> MLVSCIRRQADRRTRHHMMLDGQINPREWMNWHPKEYQPWYFDRHKFLYERQQYAHFHHLLCHQVFLKDMLHLVQHPEPYTHIVDCRTSPLKMHRWVPHSWWLPRDEVEYALQLTPDEFADMYGFHK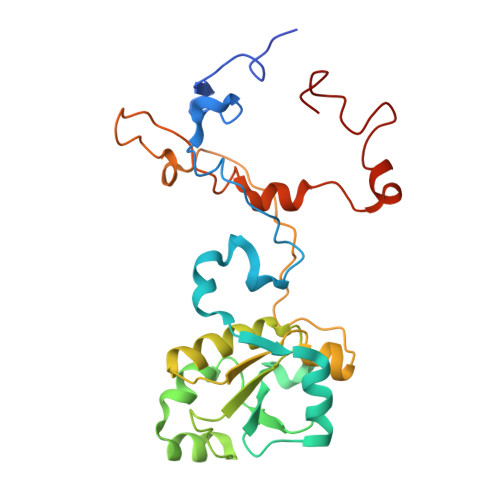PRKSDDVILVSHNGLYSEQAGWEWKKQFYQHVYNYRGGTNELFGEQYNDVALKDSLPPWKGPFPQSGIFVDKWSKRKVLTRTGPFDRQYEMQDFALPDLELERPRHPEEGPRQNMPYGLQ> ADTIVAVELDTYPNTDIGDPSYPHIGIDIKSVRSKKTAKWNMQNGKVGTAHIIYNSVDKRLSAVVSYPNADSATVSYDVDLDNVLPEWVRVGLSASTGLYKETNTILSWSFTSKLKSNSTHETNALHFMFNQFSKDQKDLILQGDATTGT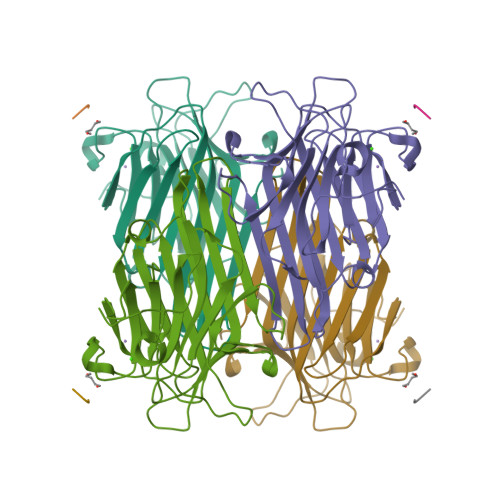DGNLELTRVSSNGSPQGSSVGRALFYAPVHIWESSAVVASFEATFTFLIKSPDSHPADGIAFFISNIDSSIPSGSTGRLLGLFPDAN;> YPY> SEFFWDVQKIQEISNVEEHSVVKCVTVNTSRLISQLNEELQDEESGVNFIVTQLQLLINNVYEKIQKSPGVPAHRSLMINLNFTRLKFSIAYWDILLERSLDLINGPSKTGARYFITEVTPVDRSRYVENNQYFLAFKANQRLTRNSVDMDEFIDFEILIKQIIFDLFKKNGIPDQDFEAILSRFHNLESLVVAF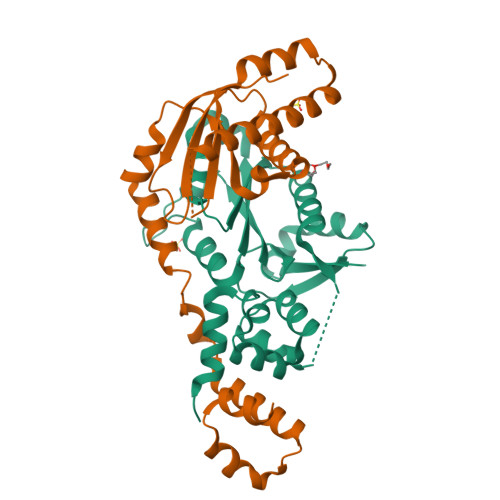NE;> ENKCIAVNENKVIENQKVIQSLCKNSHLDLIEQSYFGECDFIINHSTCVYKIQASRFMQLRNNGSLHYDKAVNDLLTEFQRVIIIVEFSEIIQDVDPDLFWKIKLYLLNSRVDVFFIHETTDFFIDWMKYFIARWAFSYNDEAAANIANADILLDLGFNILLVRKIFQTYSLEEFFMAIIKEESKAVKMLTVSQMTRLKKLLTLEW> MAEKRTGLAEDGAKSVYERLKNDRAPYETRAQNCAQYTIPSLFPKDSDNASTDYQTPWQAVGARGLNNLASKLMLALFPMQTWMRLTISEYEAKQLLSDPDGLAKVDEGLSMVERIIMNYIESNSYRVTLFEALKQLVVAGNVLLYLPEPEGSNYNPMKLYRLSSYVVQRDAFGNVLQMVTRDQIAFGALPEDIRKAVEGQGGEKKADETIDVYTHIYLDEDSGEYLRYEEVEGMEVQGSDGTYPKEACPYIPIRMVRLDGESYGRSYIEEYLGDLRSLENLQEAIVKMSMISSKVIGLVNPAGITQPRRLTKAQTGDFVTGRPEDISFLQLEKQADFTVAKAVSDAIEARLSFAFMLNSAVQRTGERVTAEEIRYVASELEDTLGGVYSILSQELQLPLVRVLLKQLQATQQIPELPKEAVEPTISTGLEAIGRGQDLDKLERCVTAWAALAPMRDD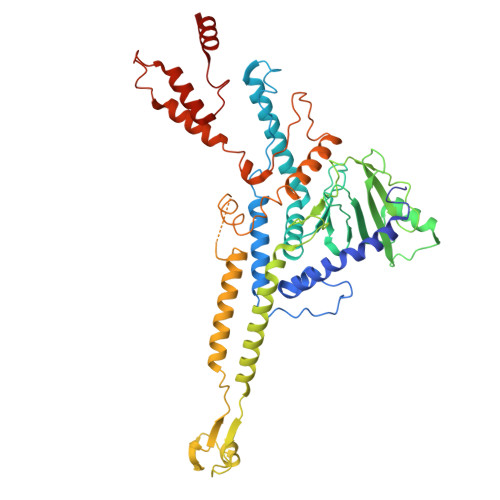PDINLAMIKLRIANAIGIDTSGILLTEEQKQQKMAQQS> YPPGYPMQAYVDPSNPNAGK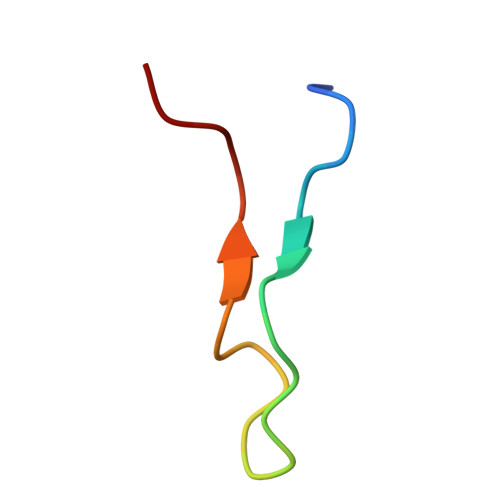VLLPTP>[8x]DDVTVVYQNGLPVISVRLPSRRERCQFTLKPISDSVGVFLRQLQEEDRGIDRVAIYSPDGVRVAASTGIDLLLLDDFKLVINDLTYHVRPPKRDLLSHENAATLNDVKTLVQQLYTTLCIEQHQLNKERELIERLEDLKEQLAPLEKVRIEISRKAEKRTTLVLWGGLAYMATQFGILARLTWWEYSWDIMEPVTYFITYGSAMAMYAYFVMTRQEYVYPEARDRQYLLFFHKGAKKSRFDLEKYNQLKDAIAQAEMDLKRLRDPLQVHLPLRQIG;>[8x]VIVTRSGAILPKPVKMSFGLLRVFSIVIPFLYVGTLISKNFAALLEEHDIFVPE;>MFRLNSLSALAELAVGSRWYHGGSQPIQIRRRLMMVAFLGASAVTASTGLLWKRAHAESPPCVDNLKSDIGDKGKNKDEGDVCNHEKKTADLAPHPEEKKKKRSGFRDRKVMEYENRIRAYSTPDKIFRYFATLKVISEPGEAEVFMTPEDFVRSITPNEKQPEHLGLDQYIIKRFDGKKISQEREKFADEGSIFYTLGECGLISFSDYIFLTTVLSTPQRNFEIAFKMFDLNGDGEVDMEEFEQVQSIIRSQTSMGMRHRDRPTTGNTLKSGLCSALTTYFFGADLKGKLTIKNFLEFQRKLQHDVLKLEFERHDPVDGRITERQFGGMLLAYSGVQSKKLTAMQRQLKKHFKEGKGLTFQEVENFFTFLKNINDVDTALSFYHMAGASLDKVTMQQVARTVAKVELSDHVCDVVFALFDCDGNGELSNKEFVSIMKQRLMRGLEKPKDMG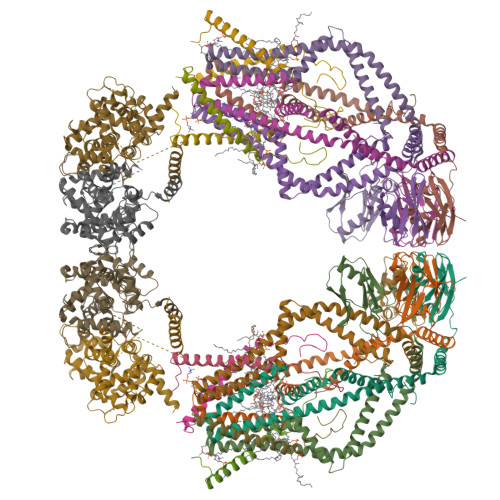FTRLMQAMWKCAQETAWDFALPKQ[2x];>PSLRKQRFMQFSSLEHEGEYYMTPRDFLFSVMFEQMERKTSVKKLTKKDIEDTLSGIQTAGCGSTFFRDLGDKGLISYTEYLFLLTILTKPHSGFHVAFKMLDTDGNEMIEKREFFKLQKIISKQDDLMTVKTNETGYQEAIVKEPEINTTLQMRFFGKRGQRKLHYKEFRRFMENLQTEIQEMEFLQFSKGLSFMRKEDFAEWLLFFTNTENKDIYWKNVREKLSAGESISLDEFKSFCHFTTHLEDFAIAMQMFSLAHRPVRLAEFKRAVKVATGQELSNNILDTVFKIFDLDGDECLSHEEFLGVLKNRMHRGLWVPQHQSIQEYWKCVKKES[2x]> MNITQAAEQAIRLWFNTPDPMQRLHMAKTIRTWIRQDKFAQVDQANMPNCVQQILNIIYDGLKPQPVQLPISYYAQLWYNLLDILRRFTFLPIISPYIHQVVQMFCPRENGPQDFRELICNLISLNWQKDPHMKHCANQVFQIFNCIIMGVKNEKLRTEFAQHLKFEKLVGTLSEYFNPQVHPGMINPAIFIIFRFIISKDTRLKDYFIWNNNPHDQPPPPTGLIIKLNAVMIGSYRLIAGQNPETLPQNPELAHLIQVIIRTFDLLGLLLHDSDAIDGFVRSDGVGAITTVVQYPNNDLIRAGCKLLLQVSDAKALAKTPLENILPFLLRLIEIHPDDEV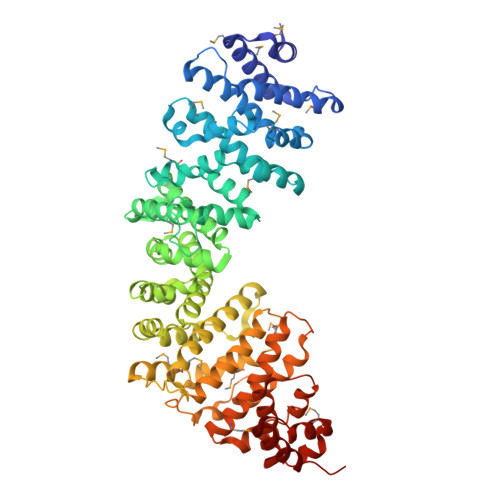IYSGTGFLSNVVAHKQHVKDIAIRSNAIFLLHTIISKYPRLDELTDAPKRNRVCEIICNCLRTLNNFLMMWIPTPNGETKTAGPNEKQQVCKFIEIDILKKLMSCLSCEGMDTPGLLELRSTILRSFILLLRTPFVPKDGVLNVIDENRKENLIGHICAAYSWVFRQPNNTRTQSTKQQLVERTISLLLVLMEQCGAEKEVAQYSYSIDCPLNLLNGNQVKPTFIHNVLVVCDKILEHCPTRADIWTIDRPMLEGLTNHRNSDIAKAANSLLSRFPEN> MAHHHHHHMSTPQLMRVKKLSEFAILPVRSSQF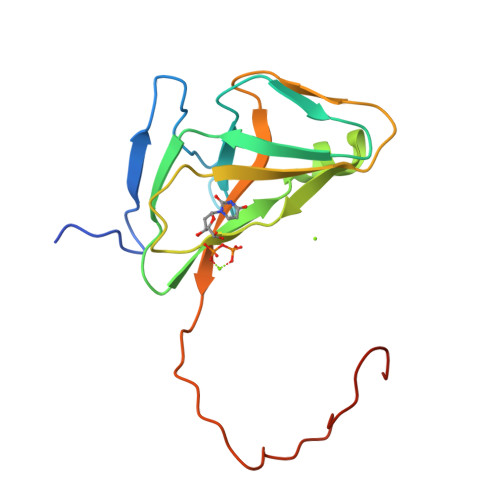AAGFDLASAYDYVVPARGKCLVKTDLAVAVPHGYYGRVAPRSGLAVKNFIDVGAGVVDSDYRGNLGVLLFNHGDEDFKIARGDRIAQFVIEQIALPDIVEVDDLDETERGAGGFGSTGVKSK4-[[4-[4-chloranyl-3-(trifluoromethyl)phenoxy]-3-cyano-phenyl]sulfamoyl]benzoic acid | C21 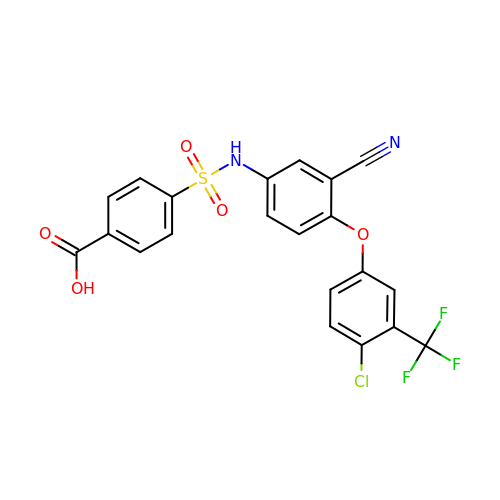H12 Cl F3 N2 O5 S | DJDKMQCYTRHYFU-UHFFFAOYSA-N6-({4-[(3,5-difluorophenyl)sulfonyl]benzyl}carbamoyl)-1-(5-O-phosphono-beta-D-ribofuranosyl)imidazo[1,2-a]pyridin-1-ium | C26 H25 F2 N3 O10 P S | 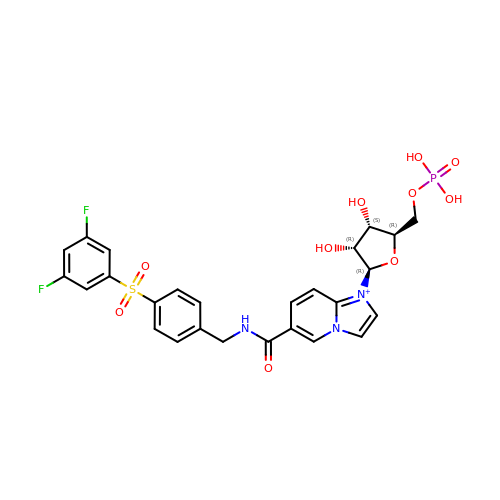ZYTGSQWLYZVDKX-IGGXFAESSA-O2-[[(3~{S})-2,5-bis(oxidanylidene)pyrrolidin-3-yl]carbamoyl]-4-nitro-benzoic acid | C12 H9 N3 O7 | 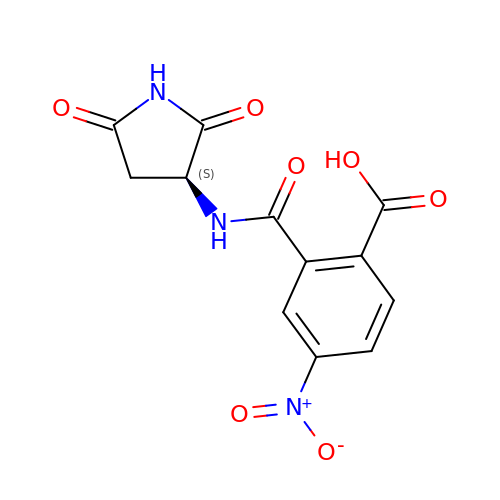QDQOIENHMXVJIB-QMMMGPOBSA-N[[(2~{R},3~{S},4~{R},5~{R})-5-(6-azanyl-2-piperazin-4-ium-1-yl-purin-9-yl)-3,4-bis(oxidanyl)oxolan-2-yl]methoxy-oxidanyl-phosphoryl]methylphosphonic acid | C15 H26 N7 O9 P2 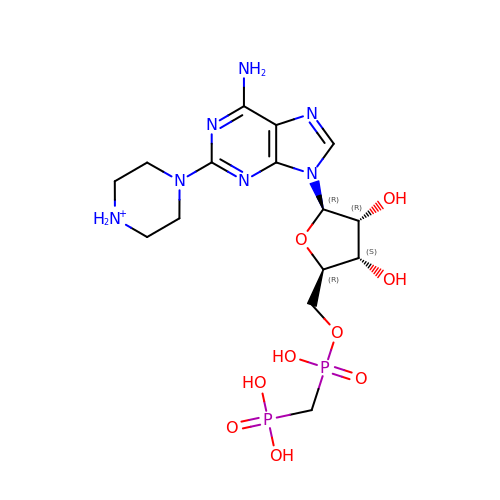| GUHCLCYLXMLIOC-IDTAVKCVSA-O> VVGGTDADEGEWPWQVSLHALGQGHICGASLISPNWLVSAAHCYIDDRGFRYSDPTQWTAFLGLHDQSQRSAPGVQERRLKRIISHPFFNDFTFDYDIALLELEKPAEYSSMVRPICLPDASHVFPAGKAIWVTGWGHTQYGGTGALILQKGEIRVIQQTTCENLLPQQITPRMMCVGFLSGGVDSCQGDSGGPLSSVEADGRIFQAGVVSWGDGCAQRNKPGVYTRLPLFRDWIKENTGV

Matriptase is a type II transmembrane serine protease that is found on the surfaces of epithelial cells and certain cancer cells. Matriptase has been implicated in the degradation of certain extracellular matrix components as well as the activation of various cellular proteins and proteases, including hepatocyte growth factor and urokinase. Matriptase activity is down-regulated by its physiological inhibitor, hepatocyte growth factor activator inhibitor-1 (HAI-1). Sunflower trypsin inhibitor-1 (SFTI-1), a cyclic peptide inhibitor originally isolated from sunflower seeds, exhibits potent inhibitory activity toward matriptase.

We have also determined the high-resolution structure of matriptase:benzamidine complex for structural comparison. In the structure of β-matriptase-N164Q complexed with benzamidine, the benzamidine binds to the specificity pocket S1 right next to the active site and is sandwiched by the segments of Ser190-Gln192 and Trp215-Gly216 as expected. Considering the high resolutions of both matriptase-benzamidine structures (1.2 Å in our structure) and the relatively small errors of structures (0.4 Å in our structure), such differences in benzamidines are significant, and indicates that S1 pocket is larger than the molecular size of benzamidine and allows movement of benzamidine inside the S1 specificity pocket. This is consistent with the observed higher temperature factor of benzamidine (40 Å2) comparing to the average temperature factor of protein (15 Å2). The point mutation removes a glycosylation site (N164) and allows the protein to be purified to homogeneity. Comparison of the conformations of matriptase in the benzamidine- and SFTI-1-bound forms reveals that they are nearly identical except the side chain of Phe99 at the S2 subsite, which will be discussed later, and Gln192 at the S3 subsite. Gln192 side chain is solvent-exposed in the benzamidine-bound structure and forms the lining of the extended active site groove.> MGSSHHHHHHSSGTGSGHMLTKEQLYQQAM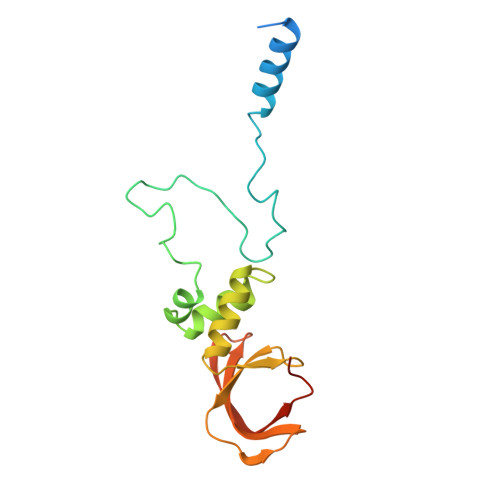EEAAWHHMPHPSDSERIRQYLPRNPCPTPPYHHQMPPPHSDTVEFYQRLSTETLFFIFYYLEGTKAQYLAAKALKKQSWRFHTKYMMWFQRHEEPKTITDEFEQGTYIYFDYEKWGQRKKEGFTFEYRYLEDRDLQ>[12x]XGEIAQATKEI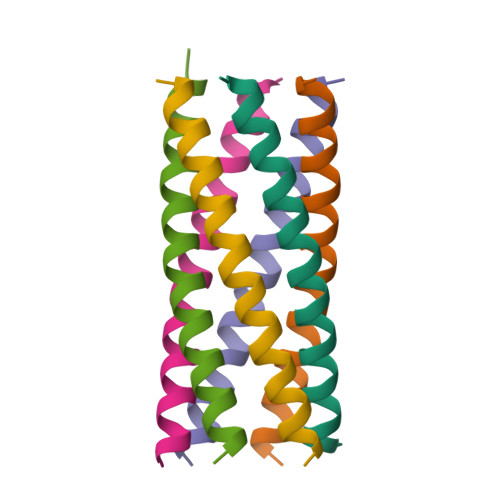AQATKEIAKATKEIAWATKEIAQATKGX> GHMATGTRYAGKVVVVTGGGRGIGAGIVRAFVNSGARVVICDKDESGGRALEQELPGAVFILCDVTQEDDVKTLVSETIRRFGRLDCVVNNAGHHPPPQRPEETSAQGFRQLLELNLLGTYTLTKLALPYLRKSQGNVINISSLVGAIGAAQAVPYVATKGAVTAMTKALALDESPYGVRVNCISPGNIWTPLWEELA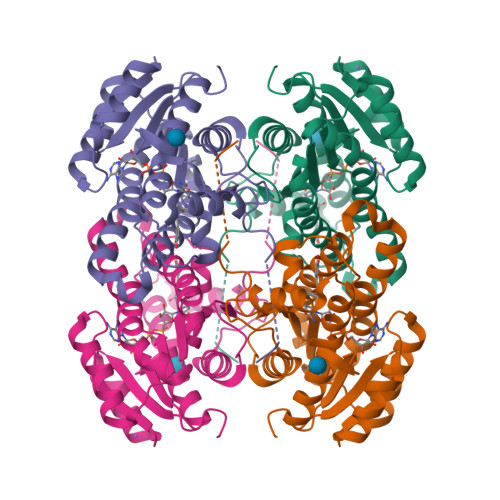ALMPDPRASIREGMLAQPLGRMGQPAEVGAAAVFLASEANFCTGIELLVTGGAELGYGCKASRSTPVDAPDIPSGS>GDSIEDKNARVIELIAAYRNRGHLMADIDPLRLDNTRFRSHPDLDVNSHGLTLWDLDREFKVDGFAGVQRKKLRDILSVLRDAYCRHVGVEYTHILEPEQQRWIQERVETKHDKPTVAEQKYILSKLNAAEAFETFLQTKYVGQKRFSLEGAETVIPMMDAVIDQCAEHGLDEVVIAMPHRGRLNVLANIVGKPYSQIFSEFEGNLNPSQAHGSGDVKYHLGATGTYIQMFGDNDIEVSLTANPSHLEAVDPVLEGLVRAKQDLLDTGEEGSDNRFSVVPLMLHGDAAFAGQGVVAETLNLALLRGYRTGGTIHIVVNNQIGFTTAPTDSRSSEYCTDVAKMIGAPIFHVNGDDPEACAWVARLAVDFRQAFKKDVVIDMLCYRRRGHNEGDDPSMTQPYMYDVIDTKRGSRKAYTEALIGRGDISMKEAEDALRDYQGQLERVFNEVRELEKHEIEPSESVEADQQIPSKLATAVDKAMLQRIGDAHLALPEGFTVHPRVRPVLEKRREMAYEGRIDWAFAELLALGSLIAEGKLVRLSGQDTQRGTFTQRHAVIVDRKTGEEFTPLQLLATNPDGTPTGGKFLVYNSALSEFAAVGFEYGYSVGNPDAMVLWEAQFGDFVNGAQSIIDEFISSGEAKWGQLSDVVLLLPHGHEGQGPDHTSGRIERFLQLWAEGSMTIAMPSTPANYFHLLRRHGKDGIQRPLIVFTPKSMLRNKAAVSDIRDFTESKFRSVLEEPMYTDGEGDRNKVTRLLLTSGKIYYELAARKAKENREDVAIVRIEQLAPLPRRRLAETLDRYPNVKEKFWVQEEPANQGAWPSFGLTLPEILPDHFTGLKRISRRAMSAPSSGSSKVHAV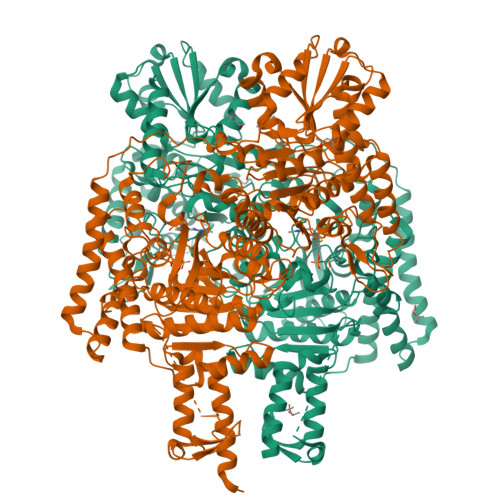EQQEILDTAFG[2x]>[6x]AKLVFFAEACIIGCMV

Oligomers of the β-amyloid peptide (Aβ) contribute to neurodegeneration in Alzheimer’s disease and are promising targets for therapies against Alzheimer’s disease. β-hairpins have emerged as important structural motifs in Aβ oligomers and have also been identified as a component of Aβ fibrils (77–86). β-hairpins are the simplest antiparallel β-sheet, comprising two hydrogen-bonded β-strands connected by a loop. 2AT is composed of β-hairpin peptides that mimic an Aβ17–36 β-hairpin, while KLT is composed of β-hairpin peptides that mimic an Aβ16–36 β-hairpin.

We have now designed and synthesized the covalently stabilized triangular trimer KLT, which mimics a triangular trimer formed by KLM. To stabilize KLM into a triangular trimer and thus create KLT, we mutated A30 and L34 to cysteine to create KLMCC and then oxidized KLMCC in aqueous DMSO to introduce disulfide cross-links. The X-ray crystallographic phases for KLT were determined by first synthesizing a variant of KLT with a para-iodo group on F19 (KLTI) and using SAD phasing to determine the structure of KLTI and then using the structure of KLTI as a search model in molecular replacement. This approach succeeded in determining the phases for KLT because the crystal structure of KLTI has the same space group and unit cell dimensions as the crystal structure of KLT.>AVKYYTLEEIQKHNNSKSTWLILHYKVYDLTKFLEEHPGGEEVLREQAGGDATENWEDVGHSTDARELSKTFIIGE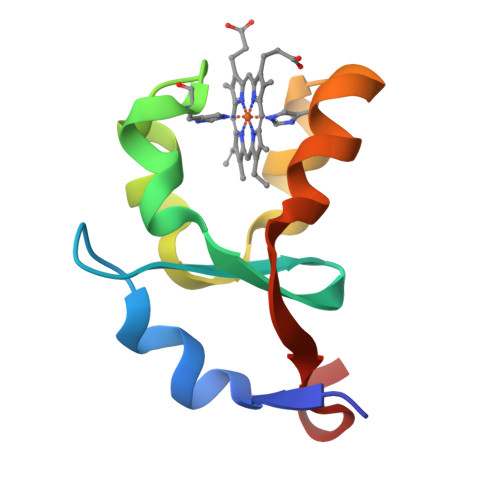LHPDDR[6x]>[8x]MEHNKSVHWSIVYRQL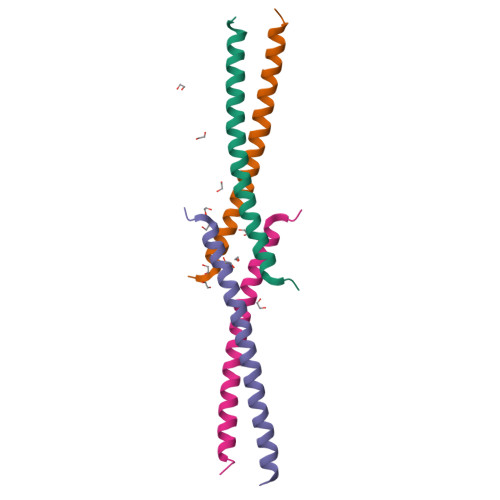GNLLEQYEVEIARLKSQLVLEKKLRIQVEKEMESVKTKQIS> EDEPEIPLSPR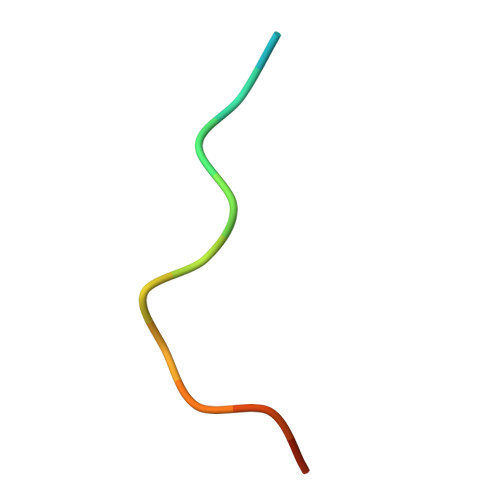PRP> GAMDPEFTIKAIKARQIYDSRGNPTVEVDLTTELGLFRAAVPSGASTGVHEALELRDNDKANY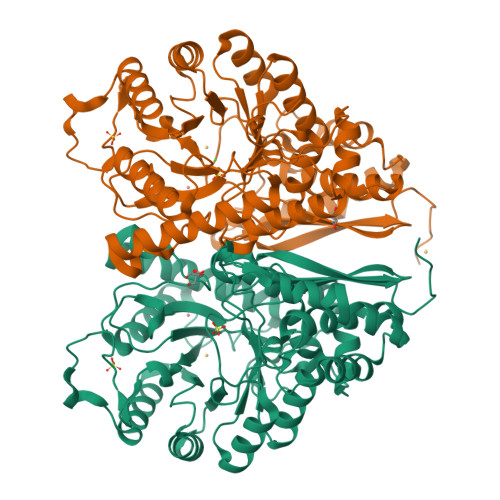HGKSVLKAVGHVNDTLGPELIKANLDVVDQASIDNFMIKLDGTENKSKFGANAILGVSLAVAKAGAAKKGVPLYKHIADLAGNKEIILPVPAFNVINGGSHAGNKLAMQEFMILPTGATSFTEAMKMGSEVYHHLKNVIKAKFGLDATAVGDEGGFAPNIQSNKEALNLISDAIAKAGYTGKIEIGMDVAASEFYKDGQYDLDFKNEKSDKSQWLPADKLANLYQEFIKDFPIVSIEDPFDQDHWEAWSNLTGCTDIQIVGDDLTVTNPKRIATAVEKKACNCLLLKVNQIGTVTESIAAHLLAKKNGWGTMVSHRSGETEDSFIGDLVVGLSTGQIKTGAPCRSERLAKYNQILRIEEEIGAGVKFAGKSFRKPQ7-[3-(aminomethyl)-4-ethoxyphenyl]-4-methylquinolin-2-amine | C19 H21 N3 O | 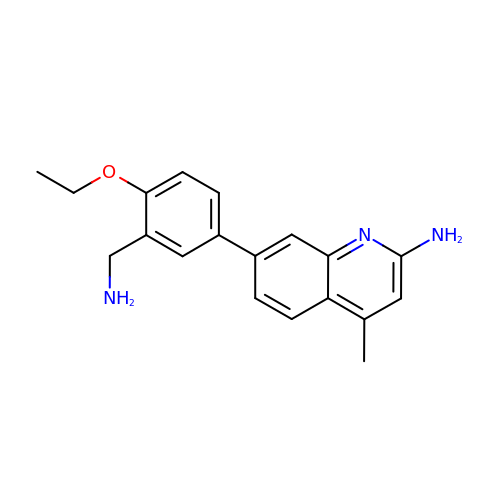AGWWSGQCTLAMKS-UHFFFAOYSA-N>MAGAIENARKEIKRISLEDHAESEYGAIYSVSGPVVIAENMIGCAMYELVKVGHDNLVGEVIRIDGDKATIQVYEETAGLTVGDPVLRTGKPLSVELGPGLMETIYDGIQRPLKAIKEESQSIYIPRGIDTPALDRTIKWQFTPGKFQVGDHISGGDIYGSVFENSLISSHKILLPPRSRGTITWIAPAGEYTLDEKILEVEFDGKKSDFTLYHTWPVRVPRPVTEKLSADYPLLTGQRVLDALFPCVQGGTTCIPGAFGCGKTVISQSLSKYSNSDAIIYVGCGERGNEMAEVLMEFPELYTEMSGTKEPIMKRTTLVANTSNMPVAAREASIYTGITLAEYFRDQGKNVSMIADSSSRWAEALREISGRLGEMPADQGFPAYLGAKLASFYERAGKAVALGSPDRTGSVSIVAAVSPAGGDFSDPVTTATLGITQVFWGLDKKLAQRKHFPSINTSVSYSKYTNVLNKFYDSNYPEFPVLRDRMKEILSNAEELEQVVQLVGKSALSDSDKITLDVATLIKEDFLQQNGYSTYDAFCPIWKTFDMMRAFISYHDEAQKAVANGANWSKLADSTGDVKHAVSSSKFFEPSRGEKEVHGEFEKLLSTMQERFAESTDDYKDHDGDYKDHDIDYKDDDDK[3x];>MVLSDKELFAINKKAVEQGFNVKPRLNYNTVSGVNGPLVILEKVKFPRYNEIVNLTLPDGTVRQGQVLEIRGDRAIVQVFEGTSGIDVKKTTVEFTGESLRIPVSEDMLGRIFDGSGRPIDNGPKVFAEDYLDINGSPINPYARIYPEEMISTGVSAIDTMNSIARGQKIPIFSASGLPHNEIAAQICRQAGLVRPTKDVHDGHEENFSIVFAAMGVNLETARFFKQDFEENGSLERTSLFLNLANDPTIERIITPRLALTTAEYLAYQTERHVLTILTDMSSYADALREVSAAREEVPGRRGYPGYMYTDLSTIYERAGRVEGRNGSITQIPILTMPNDDITHPIPDLTGYITEGQIFVDRQLHNKGIYPPINVLPSLSRLMKSAIGEGMTRKDHGDVSNQLYAKYAIGKDAAAMKAVVGEEALSIEDKLSLEFLEKFEKTFITQGAYEDRTVFESLDQAWSLLRIYPKEMLNRISPKILDEFYDRARDDADEDEEDPDTRSSGKKKDASQEESLI[3x];>MSSAITALTPNQVNDELNKMQAFIRKEAEEKAKEIQLKADQEYEIEKTNIVRNETNNIDGNFKSKLKK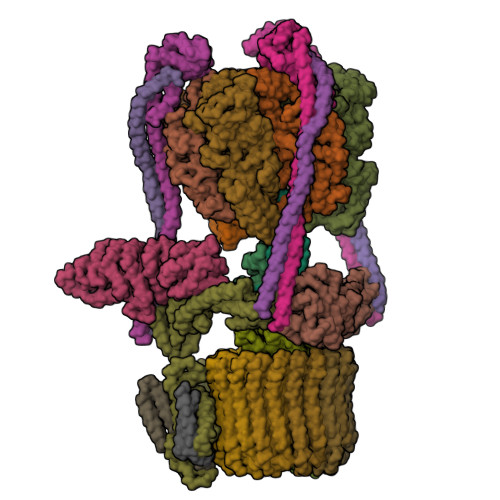AMLSQQITKSTIANKMRLKVLSAREQSLDGIFEETKEKLSGIANNRDEYKPILQSLIVEALLKLLEPKAIVKALERDVDLIESMKDDIMREYGEKAQRAPLEEIVISNDYLNKDLVSGGVVVSNASDKIEINNTLEERLKLLSEEALPAIRLELYGPSKTRKFFD[3x];>MSQKNGIATLLQAEKEAHEIVSKARKYRQDKLKQAKTDAAKEIDSYKIQKDKELKEFEQKNAGGVGELEKKAEAGVQGELAEIKKIAEKKKDDVVKILIETVIKPSAEVHINAL[3x];> MSGNREQVFPTRMTLGLMKTKLKGANQGYSLLKRKSEALTKRFRDITKRIDDAKQKMGRVMQTAAFSLAEVSYATGENIGYQVQESVSTARFKVRARQENVSGVYLSQFESYIDPEINDFRLTGLGRGGQQVQRAKEIYSRAVETLVELASLQTAFIILDEVIKVTNRRVNAIEHVIIPRTENTIAYINSELDELDREEFYRLKKVQEKKQNETAKLDAEMKLKRDRAEQDASEVAADEEPQGETLVADQEDDVIF;> MAEKRTLIAVIADEDTTTGLLLAGIGQITPETQEKNFFVYQEGKTTKEEITDKFNHFTEERDDIAILLINQHIAENIRARVDSFTNAFPAILEIPSKDHPYDPEKDSVLKRVRKLFGE;> MATALYTANDFILISLPQNAQPVTAPGSKTDSWFNETLIGGRAFVSDFKIPEFKIGSLDTLIVESEELSKVDNQIGASIGKIIEILQGLNETSTNAYRTLPINNMPVPEYLENFQWQTRKFKLDKSIKDLITLISNESSQLDADVRATYANYNSAKTNLAAAERKKTGDLSVRSLHDIVKPEDFVLNSEHLTTVLVAVPKSLKSDFEKSYETLSKNVVPASASVIAEDAEYVLFNVHLFKKNVQEFTTAAREKKFIPREFNYSEELIDQLKKEHDSAASLEQSLRVQLVRLAKTAYVDVFINWFHIKALRVYVESVLRYGLPPHFNIKIIAVPPKNLSKCKSELIDAFGFLGGNAFMKDKKGKINKQDTSLHQYASLVDTEYEPFVMYIINL;> MGATKILMDSTHFNEIRSIIRSRSVAWDALARSEELSEIDASTAKALESILVKKNIGDGLSSSNNAHSGFKVNGKTLIPLIHLLSTSDNEDCKKSVQNLIAELLSSDKYGDDTVKFFQEDPKQLEQLFDVSLKGDFQTVLISGFNVVSLLVQNGLHNVKLVEKLLKNNNLINILQNIEQMDTCYVCIRLLQELAVIPEYRDVIWLHEKKFMPTLFKILQRATDSQLATRIVATNSNHLGIQLQYHSLLLIWLLTFNPVFANELVQKYLSDFLDLLKLVKITIKEKVSRLCISIILQCCSTRVKQHKKVIKQLLLLGNALPTVQSLSERKYSDEELRQDISNLKEILENEYQELTSFDEYVAELDSKLLCWSPPHVDNGFWSDNIDEFKKDNYKIFRQLIELLQAKVRNGDVNAKQEKIIIQVALNDITHVVELLPESIDVLDKTGGKADIMELLNHSDSRVKYEALKATQAIIGYTFK;> MNQEEAIFRSADMTYVQLYIPLEVIREVTFLLGKMSVFMVMDLNKDLTAFQRGYVNQLRRFDEVERMVGFLNEVVEKHAAETWKYILHIDDEGNDIAQPDMADLINTMEPLSLENVNDMVKEITDCESRARQLDESLDSLRSKLNDLLEQRQVIFECSKFIEVNPGIAGRATNPEIEQEERDVDEFRMTPDDISETLSDAFSFDDETPQDRGALGNDLTRNQSVEDLSFLEQGYQHRYMITGSIRRTKVDILNRILWRLLRGNLIFQNFPIEEPLLEGKEKVEKDCFIIFTHGETLLKKVKRVIDSLNGKIVSLNTRSSELVDTLNRQIDDLQRILDTTEQTLHTELLVIHDQLPVWSAMTKREKYVYTTLNKFQQESQGLIAEGWVPSTELIHLQDSLKDYIETLGSEYSTVFNVILTNKLPPTYHRTNKFTQAFQSIVDAYGIATYKEINAGLATVVTFPFMFAIMFGDMGHGFILFLMALFLVLNERKFGAMHRDEIFDMAFTGRYVLLLMGAFSVYTGLLYNDIFSKSMTIFKSGWQWPSTFRKGESIEAKKTGVYPFGLDFAWHGTDNGLLFSNSYKMKLSILMGYAHMTYSFMFSYINYRAKNSKVDIIGNFIPGLVFMQSIFGYLSWAIVYKWSKDWIKDDKPAPGLLNMLINMFLAPGTIDDQLYSGQAKLQVVLLLAALVCVPWLLLYKPLTLRRLNKNGGGGRPHGYQSVGNIEHEEQIAQQRHSAEGFQGMIISDVASVADSINESVGGGEQGPFNFGDVMIHQVIHTIEFCLNCISHTASYLRLWALSLAHAQLSSVLWDMTISNAFSSKNSGSPLAVMKVVFLFAMWFVLTVCILVFMEGTSAMLHALRLHWVEAMSKFFEGEGYAYEPFSFRAIIE;> MVFGQLYALFIFTLSCCISKTVQADSSKESSSFISFDKESNWDTISTISSTADVISSVDSAIAVFEFDNFSLLDNLMIDEEYPFFNRFFANDVSLTVHDDSPLNISQSLSPIMEQFTVDELPESASDLLYEYSLDDKSIVLFKFTSDAYDLKKLDEFIDSCLSFLEDKSGDNLTVVINSLGWAFEDEDGDDEYATEETLSHHDNNKGKEGDDDILSSIWTEGLLMCLIVSALLLFILIVALSWISNLDITYGALEKSTNPIKKNN;> MNKESKDDDMSLGKFSFSHFLYYLVLIVVIVYGLYKLFTGHGSDINFGKFLLRTSPYMWANLGIALCVGLSVVGAAWGIFITGSSMIGAGVRAPRITTKNLISIIFCEVVAIYGLIIAIVFSSKLTVATAENMYSKSNLYTGYSLFWAGITVGASNLICGIAVGITGATAAISDAADSALFVKILVIEIFGSILGLLGLIVGLLMAGKASEFQ;> MEGVYFNIDNGFIEGVVRGYRNGLLSNNQYINLTQCDTLEDLKLQLSSTDYGNFLSSVSSESLTTSLIQEYASSKLYHEFNYIRDQSSGSTRKFMDYITYGYMIDNVALMITGTIHDRDKGEILQRCHPLGWFDTLPTLSVATDLESLYETVLVDTPLAPYFKNCFDTAEELDDMNIEIIRNKLYKAYLEDFYNFVTEEIPEPAKECMQTLLGFEADRRSINIALNSLQSSDIDPDLKSDLLPNIGKLYPLATFHLAQAQDFEGVRAALANVYEYRGFLETGNLEDHFYQLEMELCRDAFTQQFAISTVWAWMKSKEQEVRNITWIAECIAQNQRERINNYISVY;> MSSFYTVVGVFIVVSAMSVLFWIMAPKNNQAVWRSTVILTLAMMFLMWAITFLCQLHPLVAPRRSDLRPEFAE;> MRPVVSTGKAWCCTVLSAFGVVILSVIAHLFNTNHESFVGSINDPEDGPAVAHTVYLAALVYLVFFVFCGFQVYLARRKPSIELR;>[8x]MTELCPVYAPFFGAIGCASAIIFTSLGAAYGTAKSGVGICATCVLRPDLLFKNIVPVIMAGIIAIYGLVVSVLVCYSLGQKQALYTGFIQLGAGLSVGLSGLAAGFAIGIVGDAGVRGSSQQPRLFVGMILILIFAEVLGLYGLIVALLLNSRATQDVVC;> MSTQLASNIYAPLYAPFFGFAGCAAAMVLSCLGAAIGTAKSGIGIAGIGTFKPELIMKSLIPVVMSGILAIYGLVVAVLIAGNLSPTEDYTLFNGFMHLSCGLCVGFACLSSGYAIGMVGDVGVRKYMHQPRLFVGIVLILIFSEVLGLYGMIVALILNTRGSE>[2x]ACDYTCGSNCYSSSDVSTAQAAGYKLHEDGETVGSNSYPHKYNNWEGF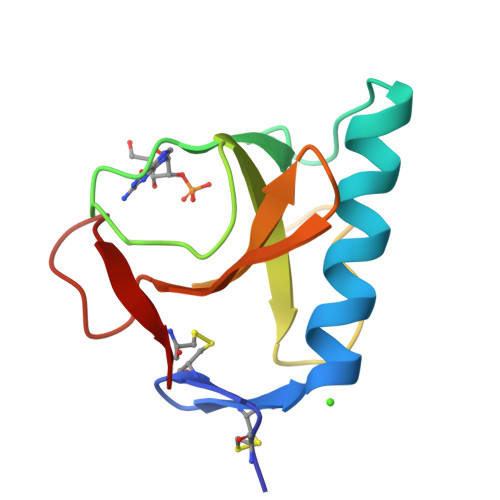DFSVSSPYYEYPILSSGDVYSGGSPGADRVVFNENNQLAGVITHTGASGNNFVECT>[6x]MSEQNTPQVREINISQEMRTSFLDYAMSVIVSRALPDVRDGLKPVHRRILYAMNDLGMTSDKPYKKSARIVGEVIGKYHPHGDSAVYESMVRMAQDFNYRYMLVDGHGNFGSVDGDSAAAMRYTEARMSKISMEILRDITKDTIDYQDNYDGSEREPVVMPSRFPNLLVNGAAGIAVGMATNIPPHQLGEIIDGVLAVSENPDITIPELMEVIPGPDFPTAGQILGRSGIRKAY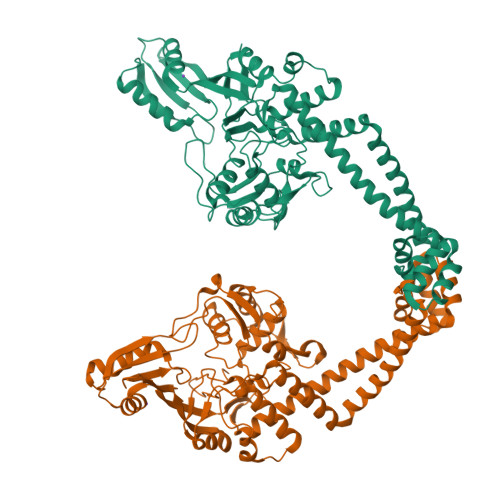ESGRGSITIRAKAEIEQTSSGKERIIVTELPYQVNKAKLIEKIADLVRDKKIEGITDLRDESDRTGMRIVIEIRRDANANVILNNLYKQTALQTSFGINLLALVDGQPKVLTLKQCLEHYLDHQKVVIRRRTAYELRKAEARAHILEGLRVALDHLDAVISLIRNSQTAEIARTGLIEQFSLTEKQAQAILDMRLQRLTGLEREKIEEEYQSLVKLIAELKDILANEYKVLEIIREELTEIKERFNDERRTEIVTSGLETIEDEDLIE>MSFTVIIPARFASSRLPGKPLADIKGKPMIQHVFEKALQSGASRVIIATDNENVADV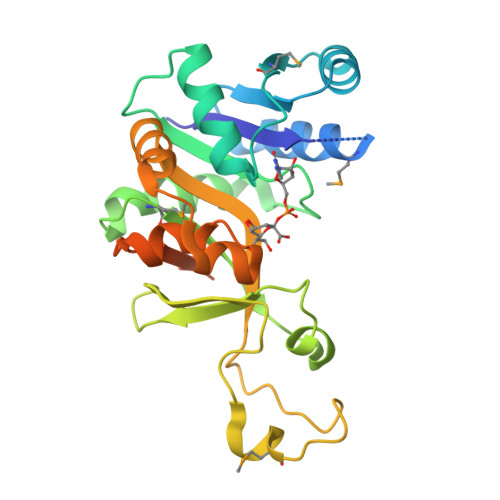AKSFGAEVCMTSVNHNSGTERLAEVVEKLAIPDNEIIVNIQGDEPLIPPVIVRQVADNLAKFNVNMASLAVKIHDAEELFNPNAVKVLTDKDGYVLYFSRSVIPYDRDQFMNLQDVQKVQLSDAYLRHIGIYAYRAGFIKQYVQWAPTQLENLEKLEQLRVLYNGERIHVELAKEVPAVGVDTAEDLEKVRAILAANGSHHHHHH[3x]>[2x]YVEFAQDFDFFYFVQQWPGSYCDTKQSCC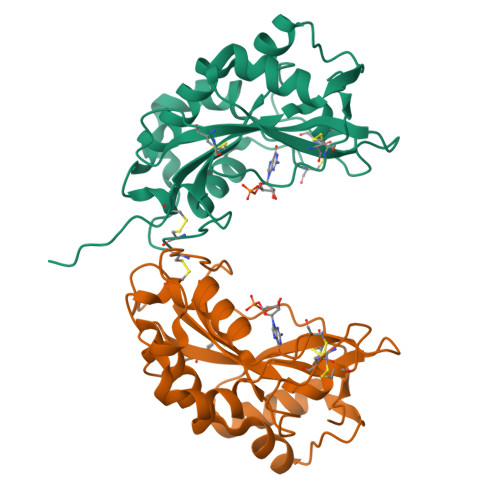YPKTGKPASDFGIHGLWPNNNDGSYPSNCDSNSPYDQSQVSDLISRMQQNWPTLACPSGTGSAFWSHEWEKHGTCAENVFDQHGYFKKALDLKNQINLLEILQGAGIHPDGGFYSLNSIKNAIRSAIGYAPGIECNVDESGNSQLYQIYICVDGSGSNLIECPIFPRGKCGSSIEFPTF>GSHMIWEQHTVTLHRAPGFGFGIAISGGRDNPHFQSGETSIVISDVLKGGPAEGQLQENDRVAMVNGVSMDNVEHAFAVQQL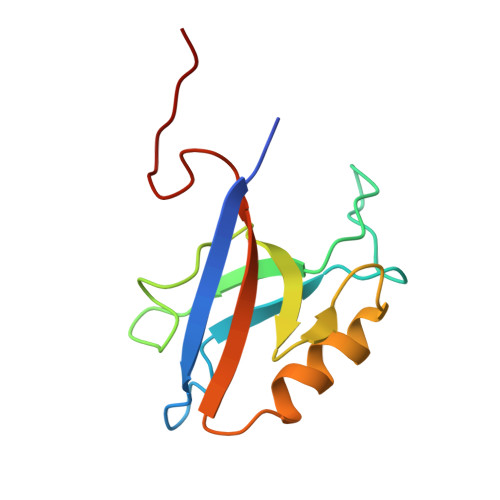RKSGKNAKITIRRKKGGGYSLTGYV[2x]>MACVNEPSPKLQKLDRNGIHGDSSPSPFFKVKKLSEKAVIPTRGSPLSAGYDLSSAVDSKVPARGKALIPTDLSIAVPEGTYARIAPRSGLAWKHSIDVGAGVIDADYRGPVGVILFNHSDADFEVKFGDRIAQLIIEKIVTPDVVEVDDLDETVRGDGGFGSTGV[3x]

Deoxyuridine triphosphate nucleotidohydrolase (dUTPase; EC 3.6.1.23) is an important enzyme that prevents uracil misincorporation during de novo DNA synthesis. It catalyzes the hydrolysis of dUTP to deoxyuridine monophosphate (dUMP) and inorganic pyrophosphate, thereby maintaining an appropriate level of dUTP with respect to deoxythymidine triphosphate (dTTP) levels. Homo-trimeric dUTPases have three active sites, each of which consists of five conserved motifs. We found that Arabidopsis dUTPase contains a unique tryptophan at the 93rd position, which is located between motifs 2 and 3.

In the apo Arabidopsis dUTPase, taurine was an indispensable additive for the growth of single crystals. When the active sites of both the apo and holo forms are superimposed, all of the apo active sites have three water molecules at similar locations as those commonly found in the holo form. These data suggest that the coordination of these water molecules is necessary for initial ligand binding at the active site. In the apo form, all of the tryptophan 93 side-chain coordinates were oriented upwards; thus, all of the tryptophan 93 Nε1 atoms were located away from the serine 89 Oγ. These are likely due to crystal-packing induced hydrophobic interactions with proline 46 in neighboring subunits.>SQIGLFSKICRVTIKTLHYYNKIGLLVPAYINPDNGYRFYTSDQLMKFHQIASLRQLGFTITEIVTLTQDENSCHIIERRRLEIQKQIRDMADMLSRINHYLQHKKKERIMLYQAALKEIPECIVYSKRFIVPDFSSY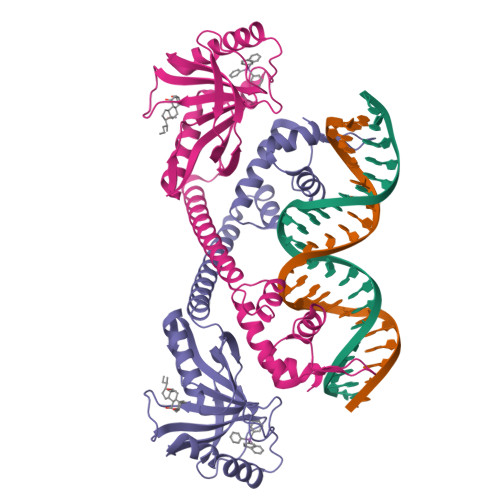IKLIPPIGQEVMKANPGLTLTTPAYCFTLYHDKEYKEKNMDVEFCEAVNDFGKNEGNIIFQVIPAITAVTVIHKGPYDSLRNAYIYLMQWVEDNGYLLTNSPRESYIDGIWNKQDSAEWMTEIQFPVEKV[2x]Unlike dyes and QDs, FPs are genetically encoded and can be particularly useful in live cell FRET imaging. In all FRET biosensors, choosing optimal FRET pairs (donor and acceptor fluorophores) are key to the high performance of biosensors in living cells. Indeed, the variety of engineered FPs with improved optical properties has made it possible to tailor FPs for FRET pairs with high FRET efficiency and develop highly sensitive FRET biosensors. Given that the chromophores of autofluorescent FPs (directly from amino acids of protein sequence) are centrally buried in the β-barrel structure with a diameter of about 2.4 nm, the effective distance for autofluorescent FP-based FRET pairs is less than 7 nm, resulting in practical maximal FRET efficiencies of 40%–55%.

With the development of two-photon FLIM (2pFLIM), FRET imaging has been extended from cultured cells to living animals. Due to the limited number of FLIM-FRET pairs, however, it has been difficult to simultaneously image two molecular events with 2pFLIM in vivo. Developing new FLIM-FRET pairs compatible with existing pairs is required. Many 2pFLIM sensors use EGFP or mEGFP as donors due to efficient FRET with RFPs and high photostability under 2P excitation, and it would be useful to develop a new FRET pair compatible with GFP-based 2pFLIM-FRET pairs that would enable imaging of multiple biochemical events in the same cell in vivo. For this purpose, a cyan-excitable orange or red FP like CyOFP1 would be a good starting point as a donor, as a single 2P excitation wavelength, for example, 940 nm, could excite both donors. CyOFP1 has an unusually high QY of 0.76 and decays as a single exponential with a long lifetime of 3.66 ns, which makes it attractive as a 2pFLIM-FRET donor, but also has some bleed-through in the emission channel for EGFP and is not fully monomeric. A red-shifted monomeric CyOFP1 paired with a far-red acceptor with high EC, for example mCardinal, could function with a GFP-based 2pFLIM-FRET pair to monitor two molecular activities simultaneously in vivo.

>[4x]MVSKGEELIKENMHSKLYLEGSVNGHQFKCTHEGEGKPYEGTQTNRIKVVEGGPLPFAFDILATMFMYGSKTFIKYPKGLPDYFKQSFPEGFTWERVMVFEDGGVLTATQDTSLQDGCLIYNVKLRGVNFPANGPVMQKKTLGWEPSTETLYPADGGLEGRCDKALKLVGGGHLHCNFKTTYRSKKPATNLKMPGVHYVDRRLERIKEADNETYVEQHEVAVARYCDLPSKLGHKLNGMDELYK[(2S)-2-[2-azanylethoxy(oxidanyl)phosphoryl]oxy-2-(13-methyltetradecanoyloxy)ethyl] 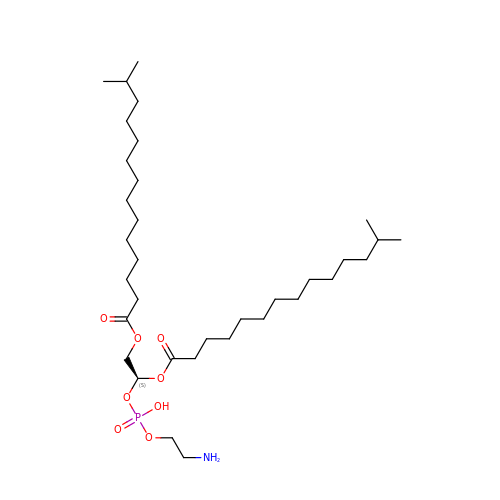13-methyltetradecanoate | C34 H68 N O8 P | TWGQVFCVUIINRS-UMSFTDKQSA-N> MHFKTKLKNRRSEVNTCLCIGLDPDEDDIKNFMKNEEQNGYKNIKNNMNSNNNGIENIIKIGKEILLTDGENIQNLSEEDKFFYFFNHFCFYIINNTKEYALVYKMNFAFYIPYGSVGINALKNVFDYLNSMNIPTMLDMKINDIGNTVKNYRKFIFEYLKSDSCTINVYMGTNMLKDICFDYEKNKYYSAYVLIKTTNKDSFIFQNELSINDKQAYIVMADETQKMATELKIEQNNEFIGFVVGSNAFEEMKIIRNKFPDSYILSPGIGAQNGDLYKTLKNGYNKDYEKLLINVGRAITKSPDPKKSSESYYN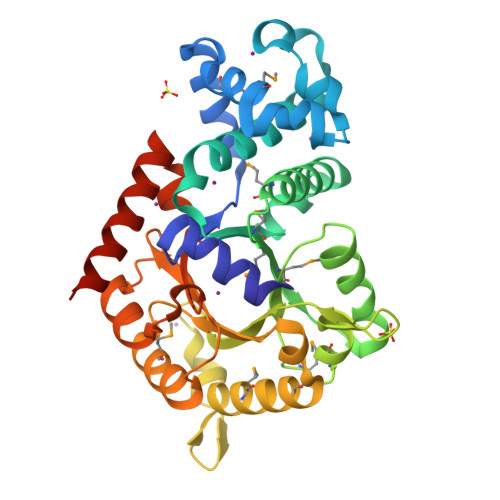QIIQIFKDIENGDNIEQV> MNDDRETPPKRKPGEDDTLFDIDFLDDTTSHSGSRSKVTNSHANANYIPPSHVLPEETIDLDADDDNIENDVHENLFMSNNHDDQTSWNANRFDSDAYQPQSLRAVKPPGLFARFGNGLKNAFTFKRKKGPESFEMNHYNAVTNNELDDNYLDSRNKFNIKILFNRYILRKNVGDAEGNGEPRVIHINDSLANSSFGYSDNHISTTKYNFATFLPKFLFQEFSKYANLFFLCTSAIQQVPHVSPTNRYTTIGTLLVVLIVSAMKECIEDIKRANSDKELNNSTAEIFSEAHDDFVEKRWIDIRVGDIIRVKSEEPIPADTIILSSSEPEGLCYIETANLDGETNLKIKQSRVETAKFIDVKTLKNMNGKVVSEQPNSSLYTYEGTMTLNDRQIPLSPDQMILRGATLRNTAWIFGLVIFTGHETKLLRNATATPIKRTAVEKIINRQIIALFTVLIVLILISSIGNVIMSTADAKHLSYLYLEGTNKAGLFFKDFLTFWILFSNLVPISLFVTVELIKYYQAFMIGSDLDLYYEKTDTPTVVRTSSLVEELGQIEYIFSDKTGTLTRNIMEFKSCSIAGHCYIDKIPEDKTATVEDGIEVGYRKFDDLKKKLNDPSDEDSPIINDFLTLLATCHTVIPEFQSDGSIKYQAASPDEGALVQGGADLGYKFIIRKPNSVTVLLEETGEEKEYQLLNICEFNSTRKRMSAIFRFPDGSIKLFCKGADTVILERLDDEANQYVEATMRHLEDYASEGLRTLCLAMRDISEGEYEEWNSIYNEAATTLDNRAEKLDEAANLIEKNLILIGATAIEDKLQDGVPETIHTLQEAGIKIWVLTGDRQETAINIGMSCRLLSEDMNLLIINEETRDDTERNLLEKINALNEHQLSTHDMNTLALVIDGKSLGFALEPELEDYLLTVAKLCKAVICCRVSPLQKALVVKMVKRKSSSLLLAIGDGANDVSMIQAAHVGVGISGMEGMQAARSADIAVGQFKFLKKLLLVHGSWSYQRISVAILYSFYKNTALYMTQFWYVFANAFSGQSIMESWTMSFYNLFFTVWPPFVIGVFDQFVSSRLLERYPQLYKLGQKGQFFSVYIFWGWIINGFFHSAIVFIGTILIYRYGFALNMHGELADHWSWGVTVYTTSVIIVLGKAALVTNQWTKFTLIAIPGSLLFWLIFFPIYASIFPHANISREYYGVVKHTYGSGVFWLTLIVLPIFALVRDFLWKYYKRMYEPETYHVIQEMQKYNISLVPRGSDSRPHVQQFQNAIRKVRQVQRMKKQRGFAFSQAEEGGQEKIVRMYDTTQKRGKYGELQDASANPFNDNNGLGSNDFESAEPFIENPFADGNQNSN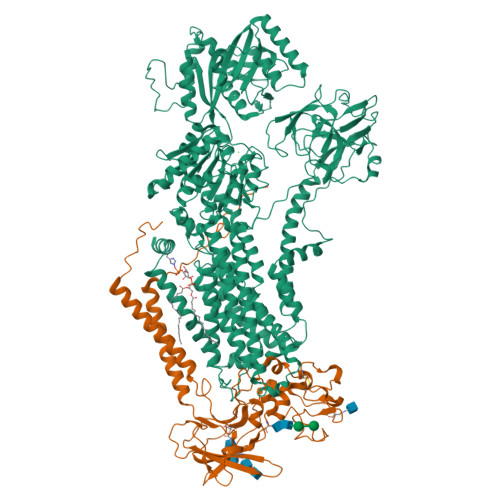RFSSSRDDISFDIGGGGLVPRGSGGTAAAPGPAPAPAPASAPAAAAPAGAGTPVTAPLAGTIWKVLASEGQTVAAGEVLLILEAMKMETEIRAAQAGTVRGIAVKAGDAVAVGDTLM;> MVSLFKRGKAPPLTKEGPTSKKPPNTAFRQQRLKAWQPILSPQSVLPLLIFVACIFTPIGIGLIVSATKVQDLTIDYSHCDTKASTTAFEDIPKKYIKYHFKSKVENKPQWRLTENENGEQSCELQFEIPNDIKKSIFIYYKITNFYQNHRRYVQSFDTKQILGEPIKKDDLDTSCSPIRSREDKIIYPCGLIANSMFNDTFSQVLSGIDDTEDYNLTNKHISWSIDRHRFKTTKYNASDIVPPPNWMKKYPDGYTDENLPDIHTWEEFQVWMRTAAFPKFYKLTLKNESASLPKGKYQMNIELNYPISLFGGTKSFVLTTNGAIGGRNMSLGVLYLIVAGLCALFGIIFLVKLIFQPRAMGDHTYLNFDDEENEDYEDVHAENTTLREILGGGGLVPRGSGGHHHHHHHHHH>[2x]MASQPNSSAKKKEEKGKNIQVVVRCRPFNLAERKASAHSIVECDPVRKEVSVRTGGLADKSSRKTYTFDMVFGASTKQIDVYRSVVCPIL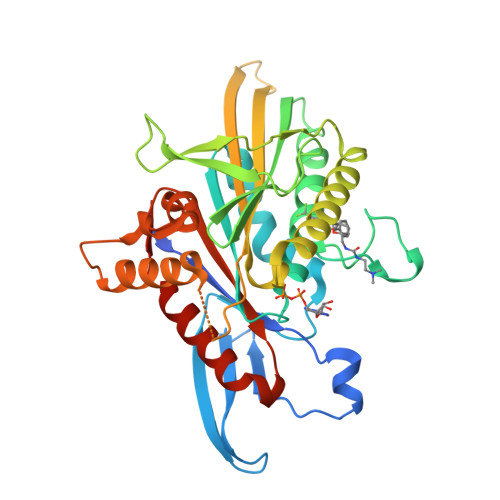DEVIMGYNCTIFAYGQTGTGKTFTMEGERSPNEEYTWEEDPLAGIIPRTLHQIFEKLTDNGTEFSVKVSLLEIYNEELFDLLNPSSDVSERLQMFDDPRNKRGVIIKGLEEITVHNKDEVYQILEKGAAKRTTAATLMNAYSSRSHSVFSVTIHMKETTIDGEELVKIGKLNLVDLAGSENIGRSGAVDKRAREAGNINQSLLTLGRVITALVERTPHVPYRESKLTRILQDSLGGRTRTSIIATISPASLNLEETLSTLEYAHRAKNILNKPEVNQK>MYIDIMPDFSPSGLLELESNNKEGIALKHVEPQDAISPDNYMDMLGLEARDRTMYELVIYRKNDKDKGPWKRYDLNGRSCYLVGRELGHSLDTDLDDRTEI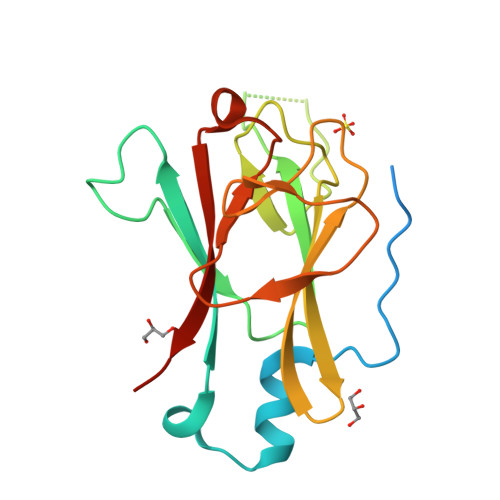VVADIGIPEETSSKQHCVIQFRNVRGILKCYVMDLDSSNGTCLNNVVIPGARYIELRSGDVLTLSEFEEDNDYELIFMNVHHHHHH[2x]> MLDAFSRAVVSADASTSTVSDIAALRAFVASGNRRLDAVNAIASNASCMVSDAVAGMICENQGLIQAGGNCYPNRRMAACLRDAEIILRYVTYALLAGDASVLDD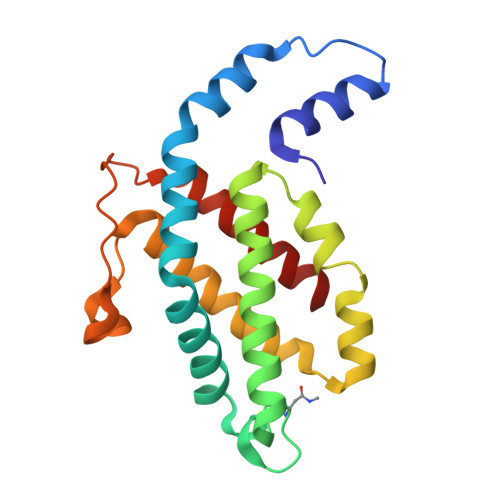RCLNGLKETYAALGVPTTSTVRAVQIMKAQAAAHIQDTPSEARAGAKLRKMGSPVVEDRCASLVAEASSYFDRVISALS> MALRGTVTDFSGFDGRADAEVLRKAMKGLGTDEDSILNLLTARSNAQRQQIAEEFKTLFGRDLVNDMKSELKGKFEKLIVALMKPSRLYDAYELKHALKGAGTDEKVLTEIIASRTPEELRAIKQAYEEEYGSNLEDDVVGDTKGYYQRMLVVLL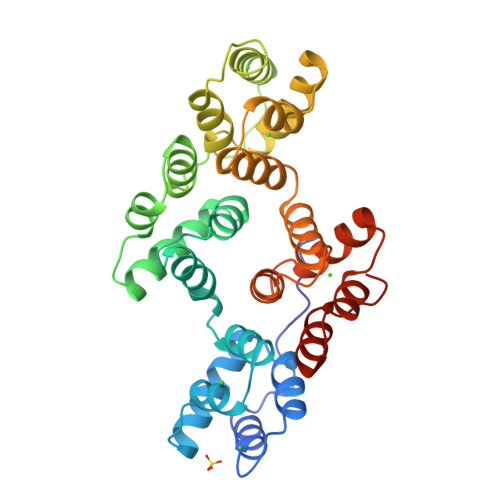QANRDPDTAIDDAQVELDAQALFQAGELKWGTDEEKFITILGTRSVSHLRRVFDKYMTISGFQIEETIDRETKGNLENLLLAVVKSIRSIPAYLAETLYYAMKGAGTDDHTLIRVIVSRSEIDLFNIRKEFRKNFATSLYSMIKGDTSGDYKKALLLLCGGEDD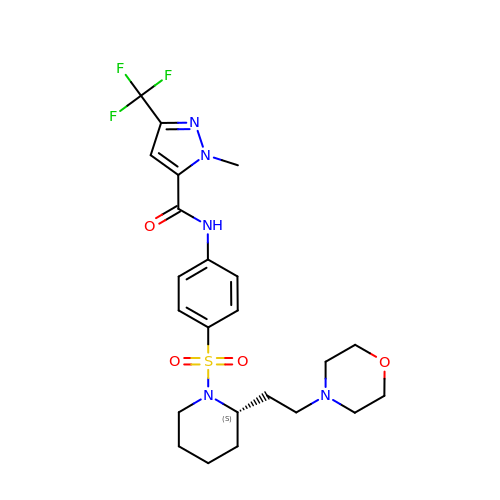2-methyl-~{N}-[4-[(2~{S})-2-(2-morpholin-4-ylethyl)piperidin-1-yl]sulfonylphenyl]-5-(trifluoromethyl)pyrazole-3-carboxamide | C23 H30 F3 N5 O4 S | JVZHTUQIMBYDSX-SFHVURJKSA-N>MEKFLVIAGPCAIESEELLLKVGEEIKRLSEKFKEVEFVFKSSFDKANRSSIHSFRGHGLEYGVKALRKVKEEFGLKITTDIHESWQAEPVAEVADIIQIPAFLCRQTDLLLAAAKTGRAVNVKKGQFLAPWDTKNVVEKLKFGGAKEIYLTERGTTFGYNNLVVDFRSLPIMKQWAKVIYDATGSVQLPGGLGDKSG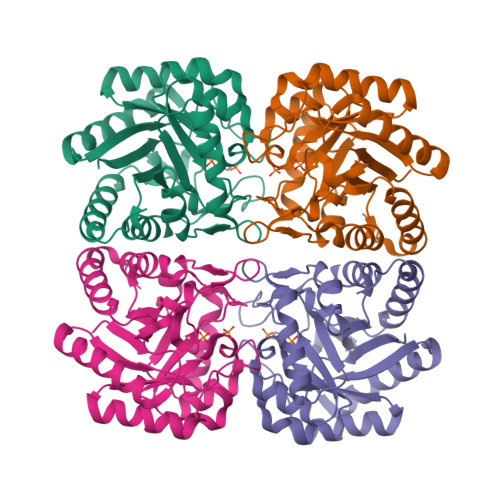GMREFIFPLIRAAVAVGCDGVFMETHPEPEKALSDASTQLPLSQLEGIIEAILEIREVASKYYETIPVK[2x]> MSERIVVDPITRIEGHLRIEAQMDGATIAQAYSSGTMVRGIETILKGRDPRDAWAFVQRICGVCTLVHGIASVRAVEDALRIELPLNAQLIRNLMIGAQYIHDHVMHFYHLHALDWVDVVSALSADPRATSELAQSISAWPKSSPGYFADTQKRIKTFVESGQLGIFANGYWGHPAYRLPPEANLMAVAHYLEALAWQRDTAKFHAIFGGKNPHPNFVVGGVPSPIDLDSDSALNAKRLAEVRNLIQSMRTFVDQVYVPDTLAIAGFYKDWGERGEGLGNFLCYGDLPTGASLDPATFLFPRGAILDRDLSTIHEVDLEATGEIQEFVNHSWYEYSVGNDRGLHPYEGQTNLEYDRRGGVAPPYKQLDVSDGYSWLKAPRWKGRSVEVGP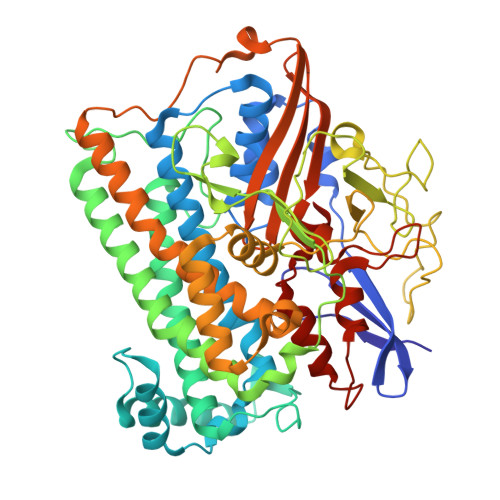LARVLMLYATGHDQARELVDSTLSRLDLPVDALYSTLGRTAARALESKILVDAMQGWYDGLIANVKSGDTKTFNETLWEPSSWPSRAQGVGIMEAPRGALGHWIVIEDGRIANYQAVVPSTWNAGPRDGRGQAGAYEAALQDNHQLVDVKQPIEILRTIHSFDPCIACAVH>[2x]MVNTEEDGLPRLIDAIEEASKIPAKRRQTPIKPTIEKLTTHLYTHGASPDSLLRLADLLTLRNHLDQASLAAITRNLYPSSTVSDEVVLRFIGALGHGQLKPTLALQALFLRWLVMVYHLLENPGVLGQVYGVLFDLLDTAAIRPQLCHLLALVTRRKHVRPFRIQAILTLSRQTGGDPNLTGLLRVFKNYYPEIIVGDATKGRASAFKHPDPQWRQHLDEIQQRRSEA;> RQKDEWAKKTSSLMKQLDWFIGEHLGAMLAAEELGGPVVGELMEIDPDDLSAGFNAHGKLKKATSQPDLDRRQRRIDDIWGPQDEQGQAHKRKRGADEALAASAEMRDLIEQLMNKLVEAGGDNSATYVEIPRESAAARFLVRSKVAMFHPNDARRLRLVDFGRDLDD;> HEAEMKSNRRRWRIMKGAASAIVAGSGIDWVRDERLRDLVLDLPD

As the core subunits of the CCAN, CENP-H, CENP-I and CENP-K (also known as Mcm16/Ctf3/Mcm22 in Saccharomyces cerevisiae and Fta3/Mis6/Sim4 in Schizosaccharomyces pombe) assemble into a ternary complex and are essential for the integrity of the kinetochore. At the inner layer, a number of centromere proteins form a network termed CCAN (the constitutive centromere-associated network) that binds to the centromere throughout the cell cycle. We here determined the crystal structures of CENP-I N-terminus alone from Chaetomium thermophilum and its complex with CENP-H/K from Thielavia terrestris, and verified the identified interactions. CENP-I integrates into the CENP-H/K complex by binding to the C-terminus of CENP-H, leading to formation of the ternary complex in which CENP-H is sandwiched between CENP-K and CENP-I. Our sequence comparisons and mutational analyses showed that this architecture of the CENP–H/I/K complex is conserved in human.

We also determined the crystal structure of the hybrid complex between ctCENP-INT and thCENP-H/K at 2.2Å with the Molecular Replacement method using the ctCENP-INT structure as start model. In one asymmetric unit of the complex crystal, one thCENP-H/K heterodimer interacts with one ctCENP-INT homodimer. The homodimer of ctCENP-INT might be a crystal packing artifact, since the complex shows a 1:1:1 stoichiometry in solution. Although the full-length thCENP-H/K proteins were used in crystallization, only the C-terminal portions of thCENP-H (184–228aa, thCENP-HCT) and thCENP-K (161–328aa, thCENP-KCT) are found in the structure. Overall, the ternary complex adopts a sandwich-like structure. ctCENP-INT and thCENP-KCT on each side pack against thCENP-HCT in the middle. thCENP-HCT contains two α-helixes HH1 and HH2 to interact with both thCENP-KCT and ctCENP-INT. In the structure of thCENP-KCT, three helixes KH1, KH2 and KH3 wrap around the HH1 helix of thCENP-HCT. On the other side of the complex, helixes α5 and α7 of ctCENP-INT contact with HH2 helix of thCENP-HCT. The sidechain of thCENP-H I205 inserts into a hydrophobic cavity surrounded by L177, F180, I270 and F300 of thCENP-K. On the other side, I211 and L219 of thCENP-H contact with the hydrophobic patch formed by W179, F180 and H184 of thCENP-K. The salt-bridge is formed between R220 in thCENP-H and E86 of ctCENP-INT. L224 in thCENP-H interacts with the hydrophobic concavity formed by L89, V126 and V130 in ctCENP-INT.>[2x]SMQRTVAHQITLLECVGKGRYGEVWRGSWQGENV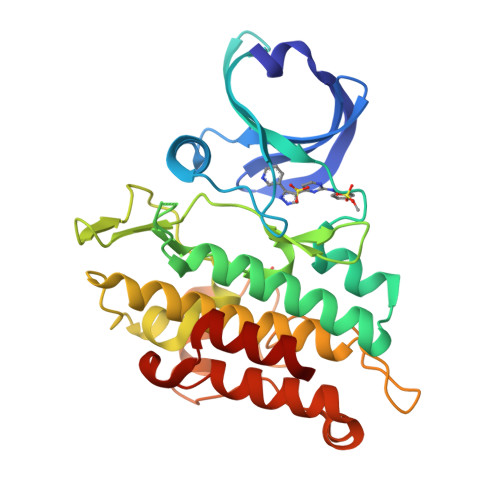AVKIFSSRDEKSWFRETELYNTVMLRHENILGFIASDMTSRHSSTQLWLITHYHEMGSLYDYLQLTTLDTVSCLRIVLSIASGLAHLHIEIFGTQGKPAIAHRDLKSKNILVKKNGQCCIADLGLAVMHSQSTNQLDVGNNPRVGTKRYMAPEVLDETIQVDCFDSYKRVDIWAFGLVLWEVARRMVSNGIVEDYKPPFYDVVPNDPSFEDMRKVVCVDQQRPNIPNRWFSDPTLTSLAKLMKECWYQNPSARLTALRIKKTLTKID> MEKLEALKISSMRPRSNILDRPLSKGKTEVSQSIVALLFSEIVQYSQSRVFTVPELQTRLHDLGQDVGTRIIDLYFVRERSSKRETKLTQMLLFVKTTVWKNLFGKEAEKLEHANDDERTYYIIEKEPLVNTFISVPKDKGSLNCAN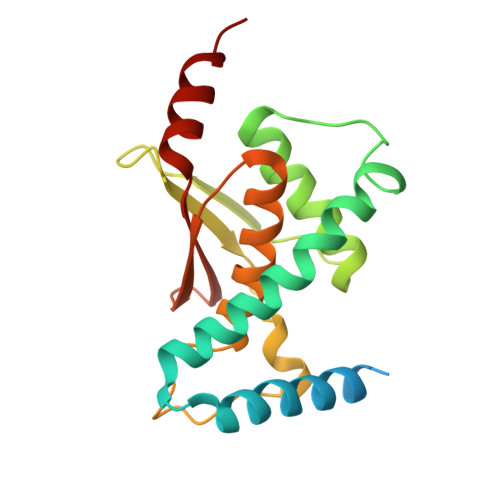FTAGIVEAVLTNCGFPCKVTAHWHKGTTYMVKFEDFVIARDKQMEEK>EGPIDKLKTPEDVPNDPLPLISDFEWSTLDIDDNLQLDELYKLLYDNYVEDIDATFRFKYSHEFFQWALKPPGWRKDWHVGVRVKSTGKLVAFIAATPVTFKLNKSNKVIDSVEINFLCIHKKLRNKRLAPVLIKEITRRVNKQNIWQALYTGGSILPTPLTTCRYQHRPINWSKLHDVGFSHLPPNQTKSSMVASYTLPNNPKLKGLRPMTGKDVSTVLSLLYKYQERFDIVQLFTEEEFKHWMLGHDENSDSNVVKSYVVEDENGIITDYFSYYLLPFTVLDNAQHDELGIAYLFYYASDSFEKPNYKKRLNELITDALITSKKFGVDVFN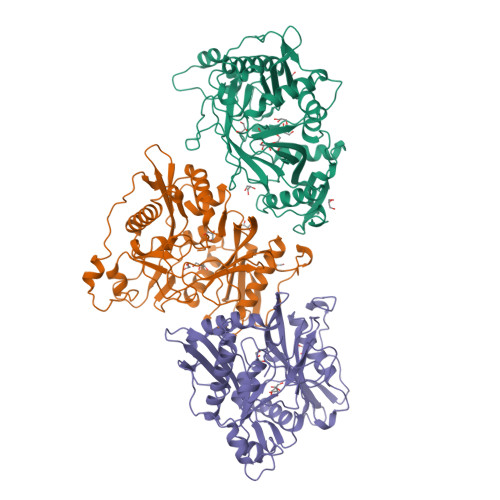CLTCQDNTYFLKDCKFGSGDGFLNYYLFNYRTFPMDGGIDKKTKEVVEDQTSGIGVVLL[3x]> RRTKLVFDDRNYSADHYLQEAKKLKHNADALSDRFEKAVYYLDAVVSFIECGNALEKNAQESKSPFPMYSETVDLIKYTMKLKNYLAPDATAADKRLTVLCLRCESLLYLRLFKLKKENALKYSKTLTEHLKNSYNNSQAPSPGLGSKAVGMPSPVSPKLSPGNSGNYSSGASSASASGSSVTIPQKIHQMAASYVQVTSNFLYATEIWDQAEQLSKEQKEFFAELDKVMGPLIFNASIMTDLVRYTRQGLHWLRQDAKLISLEHHHHHH

AFF1/4 is an intrinsic disordered scaffold protein that ties together the other components of the SEC. SEC is composed of the positive elongation factor b (P-TEFb) including cyclin-dependent kinase 9 and Cyclin T (CycT1/2), the transcription factor ELL1/210,11, the scaffold protein AFF1/47,8,10, and ENL/AF9. To release Pol II from this pause, HIV-1 trans-activator protein (Tat) recruits the super elongation complex (SEC) to the TAR RNA. Although the three binding sites of AFF4 that bind to its partners in SEC have been well defined, the structure of its C-terminal homology domain (hereafter referred to as THD) of AFF4 has not been solved.

The crystal structure of human AFF4-THD was determined by Se-SAD, and the structure was refined with native data to 2.4 Å resolution. Only one molecule of AFF-THD presents in the asymmetric unit though the AFF-THD was eluted at a volume consistent with dimer from a gel filtration column. Most residues were localized clearly, except for the highly flexible loop from G1045 to S1082 as well as the very N- and C-terminal residues. The structure of AFF-THD is comprised of eight alpha helices, of which α2, α3, α6 (Ala1116–Ala1120), α7, and α8 constitute a ring with α4 located in the center. The α1 helix, with a highly dynamic N-terminal loop standing out of the ring, packs along α2 in the manner of a helix–turn–helix fold. Together, those helices mentioned above constitute the tetratrico peptide repeat like domain (TPRL). α5 and the N-terminal portion of α6 (Gln1087 to Asn1102) sticks out of the TPRL domain, which resembles a handle of TPRL domain and is referred to as Handle Region (HR) hereafter. Although the sequence of AFF4-TPRL is not predicted as TPRs, AFF4-TPRL arranges in a fold that resembles three TPRs with α8 posing in the concave groove. In contrast, AFF4-TPRL contributes its last helix to fill the hydrophobic cleft formed by AFF4-TPRL, a novel protein fold. Though only one AFF-THD was visualized in the asymmetric unit, analytical gel filtration indicated that AFF-THD is a dimer in solution. As shown in the model, the dimerization of AFF-THD is mediated mainly by α5, and α6 (Ser1082 to T1107), as well as part of α4. Our crystal structure shows that two hydrophobic cores, with Phe1014 and Tyr1096 located in the centers, respectively, mediate the formation of an AFF4 dimer.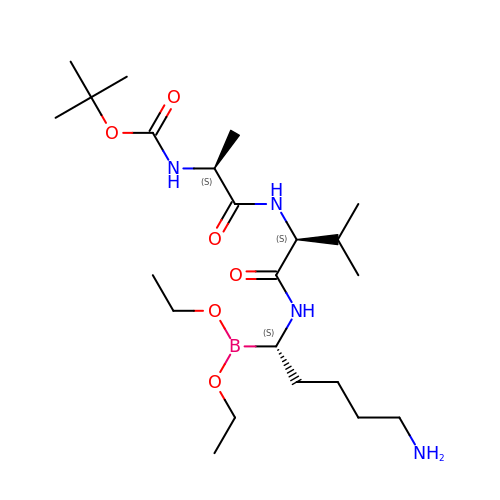N-(tert-butoxycarbonyl)-L-alanyl-N-[(1S)-5-amino-1-(diethoxyboranyl)pentyl]-L-valinamide | C22 H45 B N4 O6 | GIVAJOGGLRHKIW-BZSNNMDCSA-N>[4x]SNAVQGKAHQANK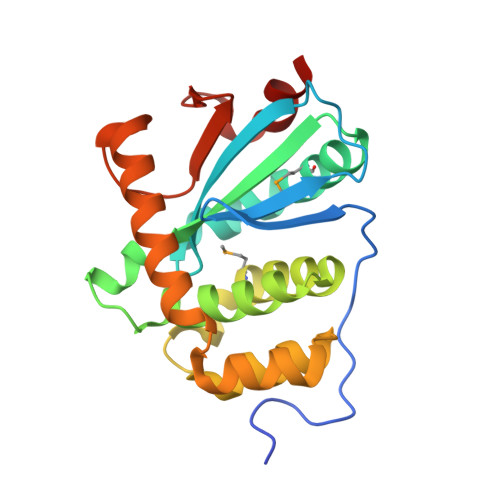YADYDKESVSFTGSVTDSAIVLKAVNAKKDAKKIDFYEDFSCPHCAELGEVTDGPMTKAIENGDIVVNLRILNFLDRDGDDGNSTKAGAAALAVAQSGDWETYWNYRALLMKEQKNIYGKWGDNDFADVAKSLGASDEVTQKIREGGAKEDFRKFAEANSKKLEKDGGSVSSPRVFIDGKEVKNGIETWVEQATS>[4x]MSIPSSQYGFVFNKQSGLNLRNDLPVHKPKAG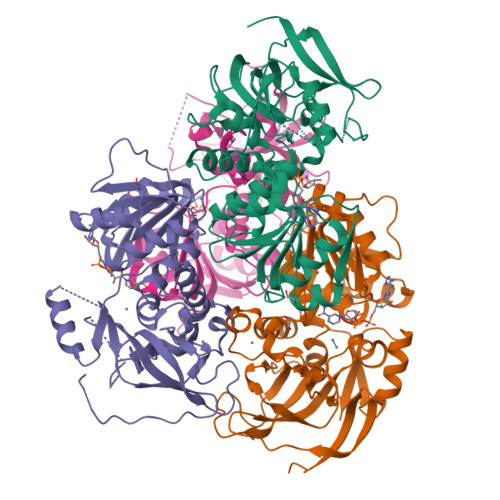QLLLKVDAVGLCHSDLHVIYEGLDCGDNYVMGHEIAGTVAAVGDDVINYKVGDRVACVGPNGCGGCKYCRGAIDNVCKNAFGDWFGLGYDGGYQQYLLVTRPRNLSRIPDNVSADVAAASTDAVLTPYHAIKMAQVSPTSNILLIGAGGLGGNAIQVAKAFGAKVTVLDKKKEARDQAKKLGADAVYETLPESISPGSFSACFDFVSVQATFDVCQKYVEPKGVIMPVGLGAPNLSFNLGDLALREIRILGSFWGTTNDLDDVLKLVSEGKVKPVVRSAKLKELPEYIEKLRNNAYEGRVVFNP> MNLEMLESQPVPEIDTLREEIDRLDAEILALVKRRAEVSKAIGKARMASGGTRLVHSREMKV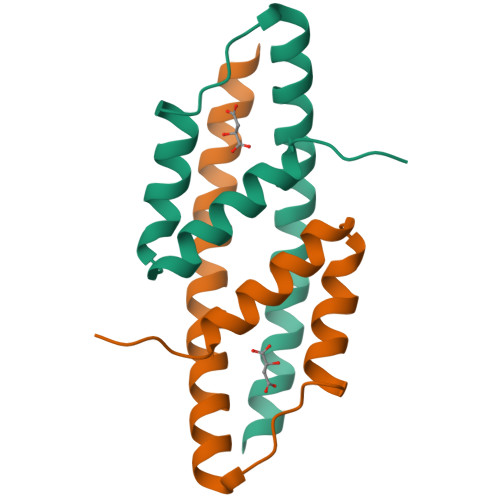IERYSELGPDGKDLAILLLRLGRGRLGH>GPAFEFAVAMMKRNSSTVKTEYGEFTMLGIYDRWAVLPRHAKPGPTILMNDQEVGVLDAKELVDKDGTNLELTLLKLNRNEKFRDIRGFLAKEEVEVNEAVLAINTSKFPNMYIPVGQVTEYGFLNLGGTPTKRMLMYNFPTRAGQAGGVLMSTGKVLGIHVGGNGHQ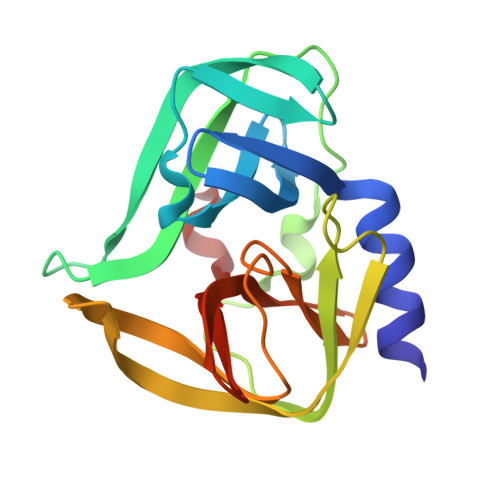GFSAALLKHYFNDEQ[2x]>[4x]HHHHHHMSMKSQFERAKIE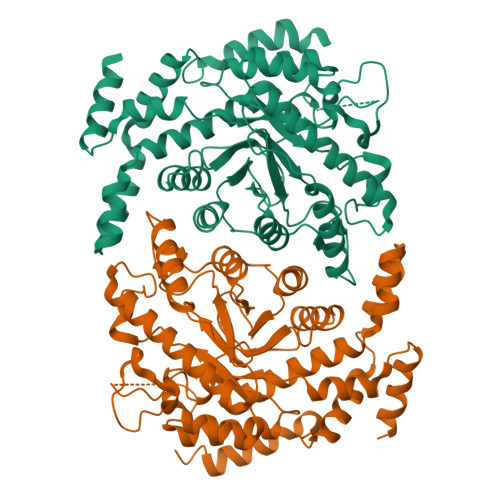YGQWGIDVEEALERLKQVPISIHCWQGDDVGGFELSKGELSGGIDVTGDYPGKATTPEELRMDLEKALSLIPGKHRVNLHAIYAETDGKVVERDQLEPRHFEKWVRWAKRHGLGLDFNPTLFSHEKAKDGLTLAHPDQAIRQFWIDHCIASRKIGEYFGKELETPCLTNIWIPDGYKDTPSDRLTPRKRLKESLDQIFAAEINEAYNLDAVESKLFGIGSESYVVGSHEFYLSYALKNDKLCLLDTGHYHPTETVSNKISAMLLFHDKLALHVSRPVRWDSDHVVTFDDELREIALEIVRNDALDRVLIGLDFFDASINRIAAWTIGTRNVIKALLFAMLIPHKQLKEWQETGDYTRRLAVLEEFKTYPLGAIWNEYCERMNVPIKEEWLKEIAIYEKEVLLQRH>[3x]MHHHHHHMILLVSPIDVEEAKEAIAGGADIIDVKNPKEGSLGANFPWMIKAIREVTPKDLLVSATVGDVPYKPGTISLAAVGAAISG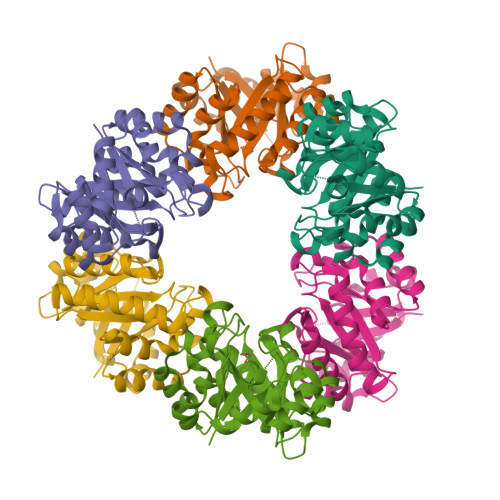ADYIKVGLYGVKNYYQAVELMKNVVRAVKDIDENKIVVAAGYADAYRVGAVEPLIVPKIARDAGCDVAMLDTAIKDGKTLFDFQSKEILAEFVDEAHSYGLKCALAGSIKKEHIPILKEIGTDIVGVRGAACKGGDRNNGRIDRELVKELKELCK>[2x]QLKTSIGLITCRMNTQNNQIETILVQKRYSLAFSEFIHCHYSINANQGHLIKMFNNMTINERLLVKTLDFDRMWYHIWIETPVYELYHKKYQKFRKNWLL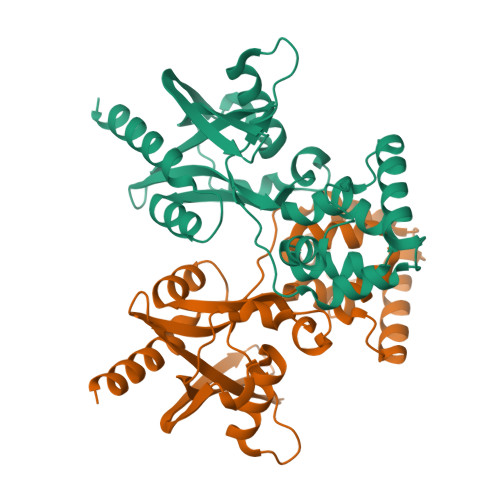PDNGKKLISLINQAKGSGTLLWEIPKGKPKEDESDLTCAIREFEEETGITREYYQILPEFKKSMSYFDGKTEYKHIYFLAMLCKSLEEPNMNLSLQYENRIAEISKISWQNMEAVRFISKRQSFNLEPMIGPAFNFIKNYLRY> GSHMSNITYVKGNILKPKSYARILIASCNCNGSWGGGIAYQLALRYPKAEKDYVEVCEKYGSNLLGKCILLPSYENSDLLICCLFTSSFGGSSHGEKQSILNYTKLALDKLKTFREAKDKTRTSEDSIGDYLNGHIKYPIGEYKLE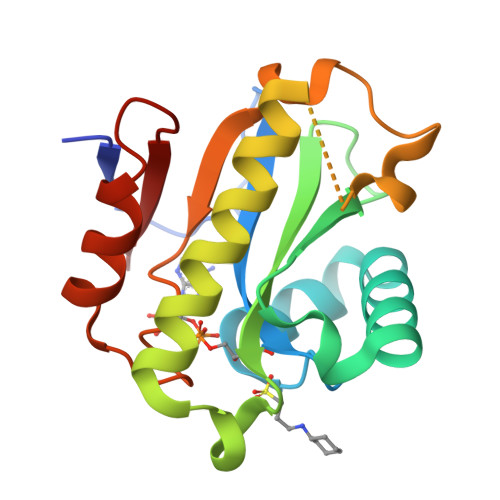MPQINSGIFGVPWKETERVLEEFSGDMSFTVYQL>[2x]MAHHHHHHMESLTLQPIARVEGTVNLPGSKSVSNRALLLAALARGTTVLTNLLDSDDVRHMLNALSALGVQYTLSADRTR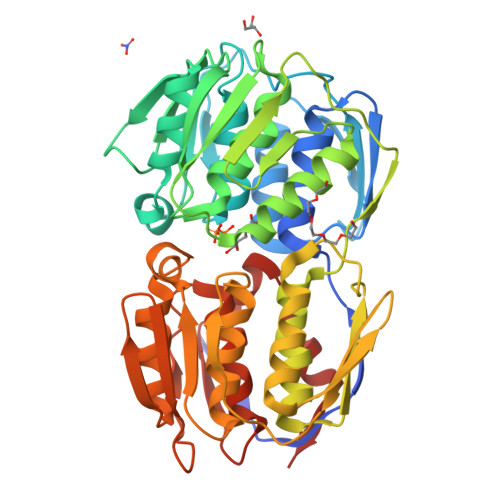CEVTGNGGPLRSAAALELFLGNAGTAMRPLAAALCLGSNDIVLTGEPRMKERPIGHLVDALRQGGAQIDCLEQENYPPLRLRGGFQGGNVEVDGSVSSQFLTALLMTAPLAPQDTVIVIKGDLVSKPYIDITLHLMKTFGVEVDNQSYQRFVVRGKQQYQSPGDYLVEGDASSASYFLAAGAIKGGTVKVTGIGRNSVQGDIRFADVLEKMGATVTWGDDFIACTHGELKAVDMDMNHIPDAAMTIATAALFAQGTTTLRNIYNWRVKETDRLFAMATELRKVGAEVEEGEDYIRITPPAKLKYAEIGTYNDHRMAMCFSLVALSDTPVTILDPKCTAKTFPDYFEQLARISTLA>SMQDPTIFEERHLKYISQLGKGNFGSVELCRYDPLGDNTGALVAVKQLQHSGPDQQRDFQREIQILKALHSDFIVKYRGVSYGPGRQSLRLVMEYLPSGCLRDFLQRHRARLDASRLLLYSSQ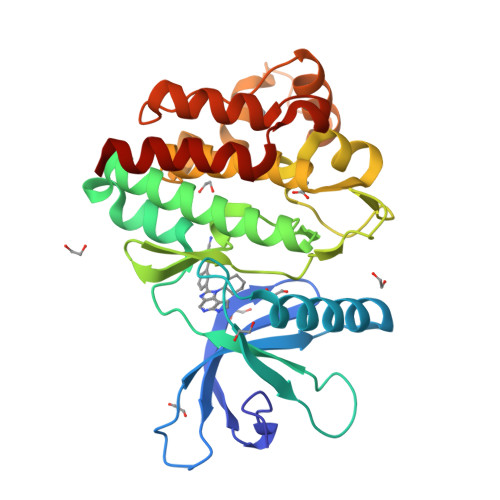ICKGMEYLGSRRCVHRALAARNILVESEAHVKIADFGLAKLLPLDKDYYVVREPGQSPIFWYAPESLSDNIFSRQSDVWSFGVVLYELFTYCDKSCSPSAEFLRMMGSERDVPALSRLLELLEEGQRLPAPPACPAEVHELMKLCWAPSPQDRPSFSALGPQLDMLWSGSR[2x]> AEVTSIPTGCNALSGKIMSGFDANRFFTGDWYLTHSRDSEVPVRCEKYQTGS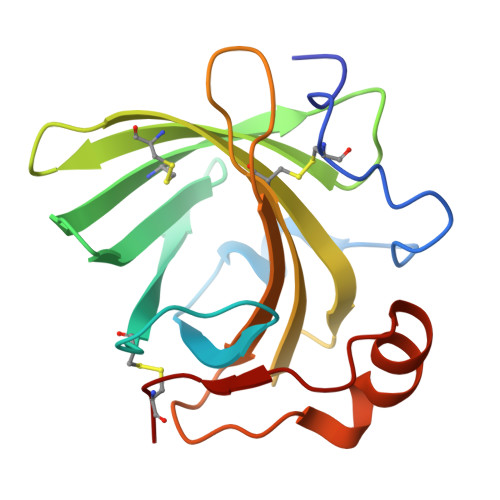NLQLNFNGKNGDVKCSGSTVSGNQGFYSFQCTTTSGGSFTSYMAVVETDYANYALLYRCGLYGSTTPKDNFLLFNRQSSGEIPAGLSTKLNQLELTSLNKLGCS>[2x]MDFYYLPGSAPCRAVQMTAAAVGVELNLKLT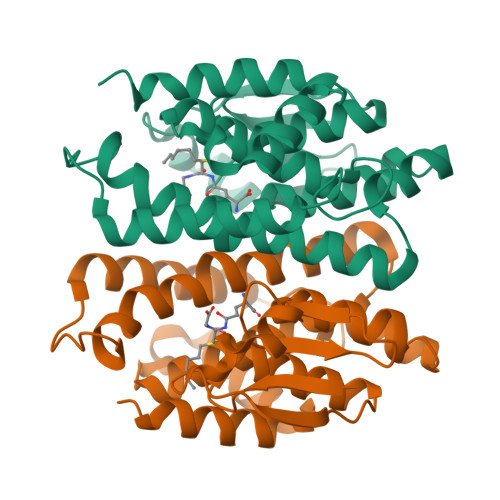NLMAGEHMKPEFLKLNPQHCIPTLVDEDGFVLWESRAIQIYLVEKYGAHDADLAERLYPSDPRRRAVVHQRLFFDVAVLYQRFAEYYYPQIFGQKVPVGDPGRLRSMEQALEFLNTFLEGEQYVAGGDDPTIADLSILATIATYEVAGYDLRRYENVQRWYERTSAIVPGADKNVEGAKVFGRYFTQK> QDAPRLTGADRPMSEVAAPPLPETI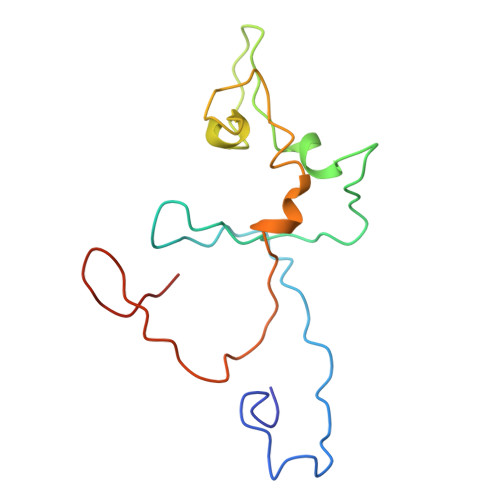TDDRRVGRNYPEQPPVIPHSIEGYQLSVNANRCLECHRRQYSGLVAAPMISITHFQDREGQMLADVSPRRYFCTACHVPQTNAQPLVTNEFRDMLTLMPASNEAE>DTYAATRYPVILVHGLAGTDKFANVVDYWYGIQSDLQSHGAKVYVANLSGFQSDDGPNGRGEQLLAYVKQVLAATGATKVNLIGHSQGGLTSRYVAAVAPQLVASVTTIGTPHRGSEFADFVQDVLKTDPTGLSSTVIAAFVNVFGTLVSSSHNTDQDALAALRTLTTAQTATYNRNFPSAGLGAPGSCQTGAATETVGGSQHLLYSWGGTAIQPTSTVLGVTGATDTSTGTLDVANVTDPSTLALLATGAVMINRASGQNDGLVSRCSSLFGQVISTSYHWNHLDEINQLLGVRGANAEDPVAVI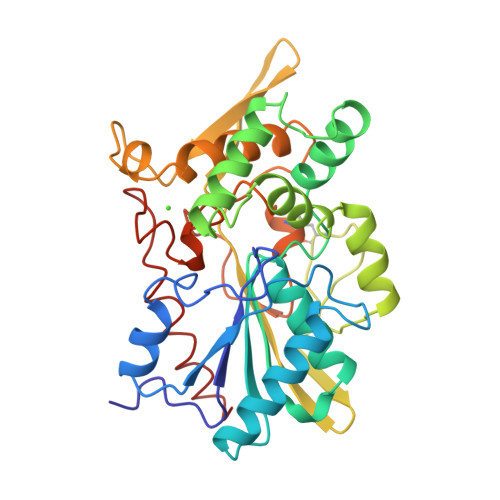RTHVNRLKLQGV[4x]>MPGSIPLIGERFPEMEVTTDHGVIKLPDHYVSQGKWFVLFSHPADFTPVSTTEFVSFARRYEDFQRLGVDLIGLSVDSVFSHIKWKEAIERHIGVRIPFPIIADPQGTVARRLGLLHAESATHTVRGVFIVDARGVIRTML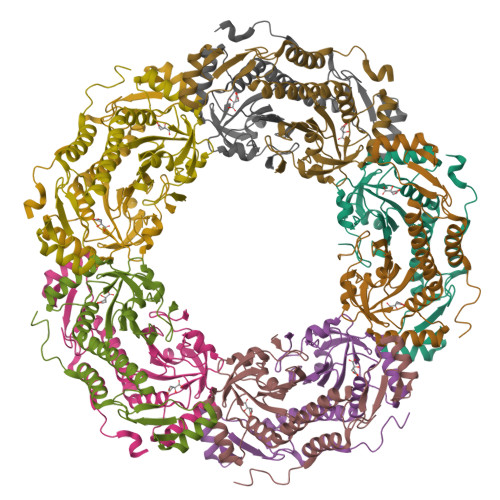YYPMELGRLVDEILRIVKALKLGDSLKRAVPADWPNNEIIGEGLIVPPPTTEDQARARMESGQYRSLDWWFSWDTPASRDDVEEARRYLRRAAEKPAKLLYEEARTHLH[10x]> DYKDDDDKLAAAQYPVVNTNYGKIRGLRTPLPNEILGPVEQYLGVPYASPPTGERRFQPPEPPSSWTGIRNTTQFAAVCPQHLDERSLLHDMLPIWFTANLDTLMTYVQDQNEDCLYLNIYVPTEDDIHDQNSKKPVMVYIHGGSYMEGTGNMIDGSILASYGNVIVITINYRLGILGFLSTGDQAAKGNYGLLDQIQALRWIEENVGAFGGDPKRVTIFGSGAGASCVSLLTLSHYSEGLFQKAIIQSGTALSSWAVNYQPAKYTRILADKVGCNMLDTTDMVECLRNKNYKELIQQTITPATYHIAFGPVIDGDVIPDDPQILMEQGEFLNYDIMLGVNQGEGLKFVDGIVDNEDGVTPNDFDFSVSNFVDNLYGYPEGKDTLRETIKFMYTDWADKENPETRRKTLVALFTDHQWVAPAVATA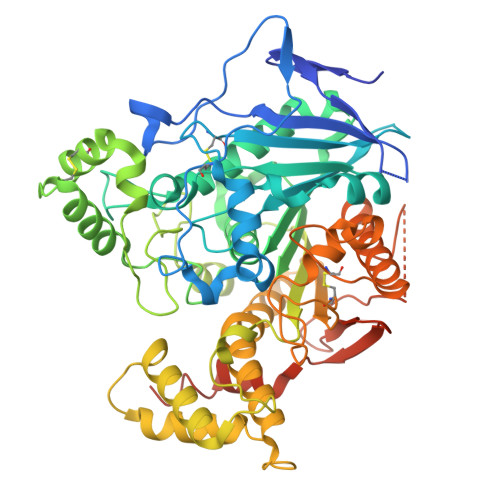DLHAQYGSPTYFYAFYHHCQSEMKPSWADSAHGDEVPYVFGIPMIGPTELFSCNFSKNDVMLSAVVMTYWTNFAKTGDPNQPVPQDTKFIHTKPNRFEEVAWSRYNPKDQLYLHIGLKPRVRDHYRATKVAFWLELVPHLHNLNEIFQYVSTTTKVPPPDMT>MGSKLINVEGGNNQDDNKYNSNNVISINNKVNKNDYFIETNKELKINLNFQNNNIISNIFSNINIYDKISNIFINNKKTYMLKYNNNINEENFFISYFEKKDDNFVPISPWHHIDLKNDDGTYNMIVEITKYNYIKLEIQLREKFNVIKQDKKKGKLRYYHNSIYWNYGALPQTYEYPKHIYQNKSKKNKEALLFTGDNDPLDILDIGSACLKIGQVVPVKILGAFTLIDEGELDWKIIAINKEDKHYEDINSLSDIEKYYPHTLSLLLEWFRSYKMADTKKLNLISKQLYDKKESEDLIMKTHHYYLEFREDVKKLKEEHSKETIKEHDYVNAQNIQFNYDKLNNNDDEPMENNLLEDINITYYKSDSAYKPDLNIWTP[5x]

The enzyme inorganic pyrophosphatase (PPase) catalyzes the hydrolysis of pyrophosphate (PPi) to inorganic phosphate (Pi). This is an exergonic reaction and can be coupled to several unfavorable and energy demanding biochemical transformations such as DNA replication, protein synthesis and lipid metabolism. Family I PPases are Mg2+ dependent enzymes known to exist as homo-hexamers in prokaryotes and dimers in eukaryotes. We report structural and biochemical characterization of these two apicomplexan PPases.

We were successful in obtaining crystals of seleno-methionine (Se-Met) labeled PfPPase and hence used single wavelength anomalous (SAD) technique to obtain the crystal structure of PfPPase. The final structure was refined to highest resolution of 3.2 Å with Rwork/Rfree of 0.22/0.27. Crystals of PfPPase belonged to space group C2 with five molecules in the asymmetric unit and Mathew’s coefficient of Vm ~ 3.0. Overall, the PfPPase crystal structure showed simple domain architecture, typified by five stranded β-barrel β4 and β7-β10. The first 36 residues of PfPPase are missing in the current crystal structure and thus the structure extends from residues 37 to 380. An interesting and a key distinct feature of PfPPase is its N region (residues 36–76) that stretches away from the structural core and is absent in both T. brucei and S. cerevisae PPases. PfPPase active site showed electron density for only one Pi molecule in two (B and C) out of five subunits (A–E) in the asymmetric unit. In structural comparisons with TbVSP1 and ScPPase, this Pi molecule in PfPPase closely corresponded to the location of Pi molecule of the bound PPi that is not directly attacked (P1). This observation suggested that the directly attacked phosphate group (P2) of the PPi was first to dissociate from the active site of PfPPase. In the asymmetric unit of PfPPase crystals, four chains formed two non-crystallographic dimers, and dimerization of the fifth monomer was mediated via the crystallographic 2-fold axis.>[2x]MATLQDIGVSAGINILSAFVFFIIFAVLRLQPFNDRVYFSKWYLKGLRSSPARGGAFAQRFVNLDFRSYMKFLNWMPEALKMPEPELIDHAGL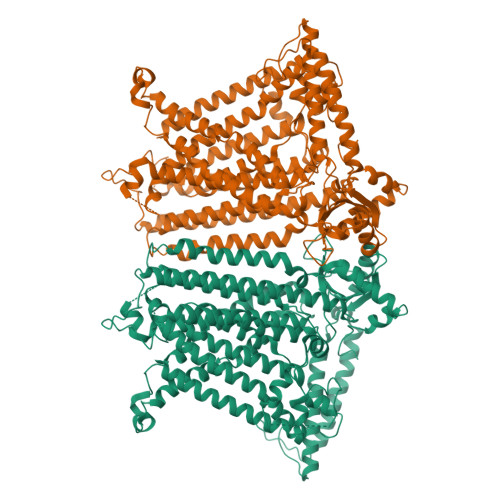DSVVYLRIYWLGLKIFTPIAVLAWAVLVPVNWTNNTLEMAKQLRNVTSSDIDKLSVSNIPEYSMRFWTHIVMAYAFTIWTCYVLMKEYETIANMRLQFVASEARRPDQFTVLVRNVPPDADESVSELVEHFFLVNHPDHYLTHQVVCNANKLADLVKKKKKLQNWLDYYQLKYARNNSQRIMVKLGFLGLWGQKVDAIEHYIAEIDKISKEISKEREEVVNDPKAIMPAAFVSFKTRWAAAVCAQTQQTRNPTQWLTEWAPEPRDVFWSNLAIPYVSLTVRRLIMHVAFFFLTFFFIVPIAFVQSLATIEGIVKAAPFLKFIVDDKFMKSVIQGFLPGIALKLFLAFLPSILMIMSKFEGFTSISSLERRAAFRYYIFNLVNVFLASVIAGAAFEQLNSFLNQSANQIPKTIGVAIPMKATFFITYIMVDGWAGVAGEILMLKPLIMFHLKNAFLVKTDKDREEAMDPGSIGFNTGEPRIQLYFLLGLVYAPVTPMLLPFILVFFALAYIVYRHQIINVYNQEYESAAAFWPDVHGRVIAALVISQLLLMGLLGTKHAALAAPFLIALPVLTIGFHHFCKGRYEPAFIRYPLQEAMMKDTLETAREPNLNLKGYLQNAYVHPVFKGDEDDYDIDDKLGKFEDEAIIVPTKRQSRRNTPAPSIISGDDSPSLPFSGKLVSNSLEVLFQ>[3x]GSAMGSASTSGNPFQANVEMKTFMERFNLTHHHQSGIYVDLGQDKEVDGTLYREPAGLCPIWGKHIELQQPDRPPYRNNFLEDVPTEKEYKQSGNPLPGGFNLNFVTPSGQRISPFPMELLEKNSNIKASTDLGRCAEFAFKTVAMDKNNKATKYRYPFVYDSKKRLCHILYVSMQLM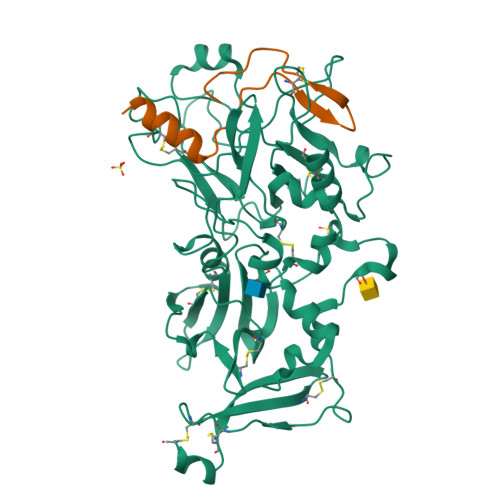EGKKYCSVKGEPPDLTWYCFKPRKSVTENHHLIYGSAYVGENPDAFISKCPNQALRGYRFGVWKKGRCLDYTELTDTVIERVESKAQCWVKTFENDGVASDQPGSGSGSGDQPHSGGVGRNYGFYYVDTTGEGKCALSDQVPDCLVSDSAAVSYTAAGSLSEETPNFIIPSNPSVTPPTPETALQCTADKFPDSFGACDVQACKRQKTSCVGGQIQSTSVDCTADEQNECGSNTAAALVPR;>GSASDITQHLNDSGLGPAVECLENLVVGPVCPAAVVAPAV[3x]> GSKKPVPIIYCNRRTGKC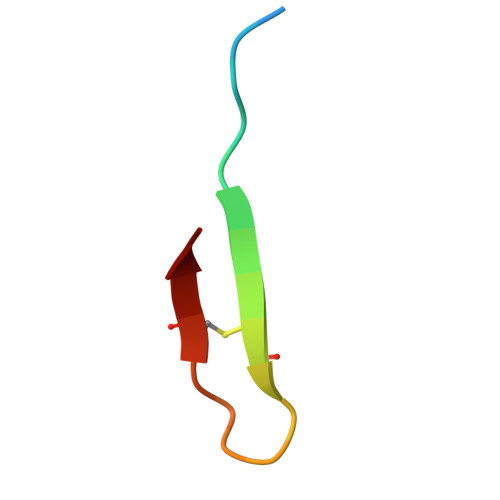QRM>MGHHHHHHMMKFINIGYGNMVSAAWIITIVSPDSAPIKRIIQDAREKGKLVDATHGRRTRAVIITDSDHVILSSV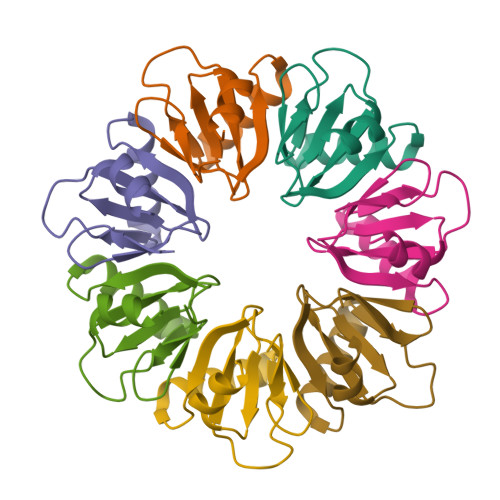QPETVANRLYGSDDFSEEG[7x]> GAAVNGSSMEPTLHNNDRLWVTSIKKPQRFDIIA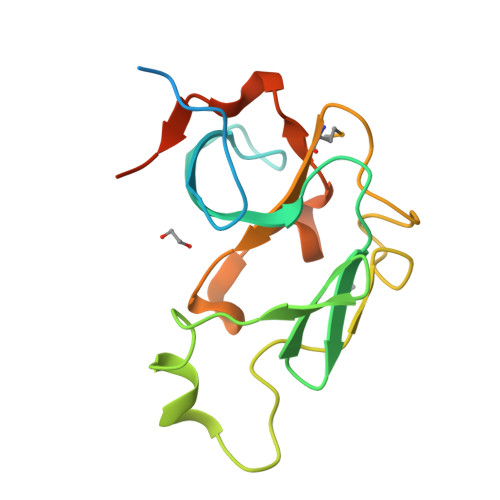FPSPRNGQRVAKRLIGLPGETVEYRDDTLYINGVSLSEDYLASAKRNVSKNENYTQDFTLETLEATQSLTVPEGMYFVLGDNRPRSDDSRYFGFVKQASVEGVLTFRYYPLDKIGFP>[4x]AEAGITGTWYNQLG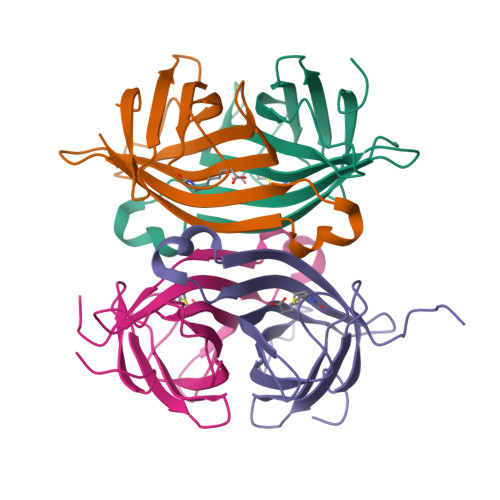ATFIVTAGADGALTGTYESAVGNAESRYVLTGRYDSAPATDGSGTALGWTVAWKNNYRNAHSATTWSGQYVGGAEARINTQWLLTSGTTEANAWKSTLVGHDTFTKVKPSAAS>HHHHHHMRVSFMVAMDENRVIGKDNNLPWRLPSELQYVKKTTMGHPLIMGRKNYEAIGRPLPGRRNIIVTRNEGYHVEGCEVAHSVEEVFELCKNEEEIFIFGGAQIFDLFLPYVDKLYITKIHHAFEGDTFFPEMDMTNWKEVFVEKGLTDEKNPYT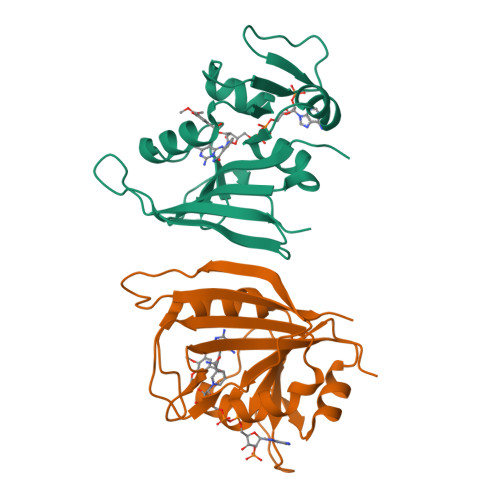YYYHVYEKQQ[2x]> HHHHHHIEGRDEEFSDMLRLIDYNKAALSKFKQDVESALHVFKTTVNSLISDQLLMRNHLRDLMGVPYCN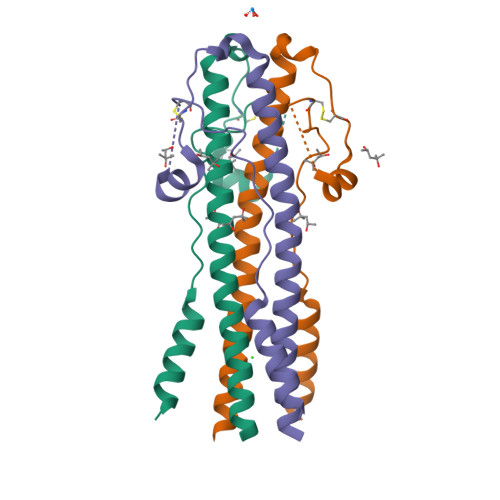YSKFWYLEHAKTGETSVPKCWLVTNGSYLNETHFSDQIEQEADNMITEMLRKDYIKRQGSTPLALMD> SNATLGKET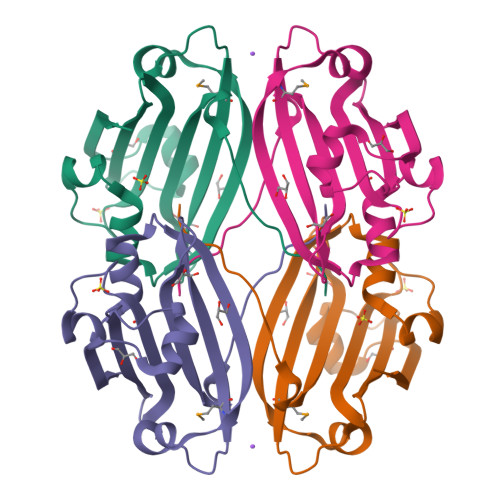KTTVHKFGLEPPSELIQKQLRANLDDDIWEVIRSRKIDGEHVILDKDYFFRKHVPHLTKEICENSIYEYIEGELGLSISYAQKEIVAEPCTDEDRELLDLRGYDHMVVVRNYVFLEDTSLFQYTESRHRLDKFRFVDFARRGK>DGANSDAAKEYLTKDSFSYEVYGIIAMQAAYRDYDSGDAKQDDNLGGMQLNNESRIGFRGKKQFANFEPTFIWQIEGGYVDPSFGGEGAGLGERDTFVGFESASWGQVRLGRVLTPMYELVDWPASNPGLGDVYDWGGAIGGAKYQDRQSNTIRWDSPMYADKFSIDAAVGAGDKAGLGAGDDYWGGIAAHYKLGPLQLDAAYEGNRNIEAEGQTWENNTYLVGVQGWFENGISFFAQYKYMEADASNGVNEKQDAMSAGLMYTTGDWQYKLGYAANFDLERDGKTLSNTSDDVVSAQIMYFVDPSAVLYAR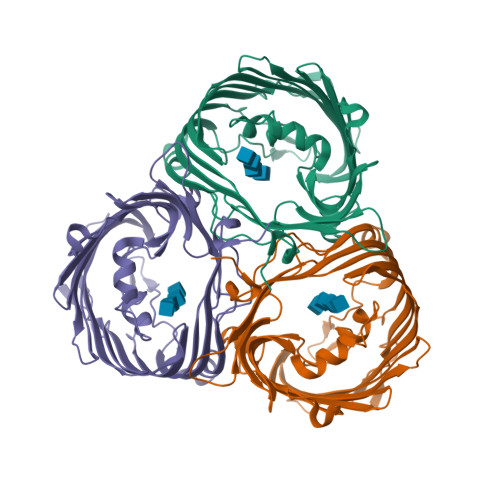ARMNDFNEGLDGLDDAARWTSGTNGDYNEYSVGVEYYF[3x]>MRTIHANSSAVREDHRALDVATELAKTFRVTVRERERAGGTPKAERDAIRRSGLLTLLISKERGGLGESWPTVYEAIAEIASADASLGHLFGYHFSNFAYVDLFASPEQKARWYPQAVRERWFLGNASSENNAHVLDWRVTATPLPDGSYEINGTKAFCSGSADADRLLVFAVTSRDPNGDGRIVAALIPSDRAGVQVNGDWDSLGMRQTDSGSVTFSGVVVYPDELLGTPGQVTDAFASGSKPSLWTPITQLIFTHLYLGIARGALEEAAHYSRSHSR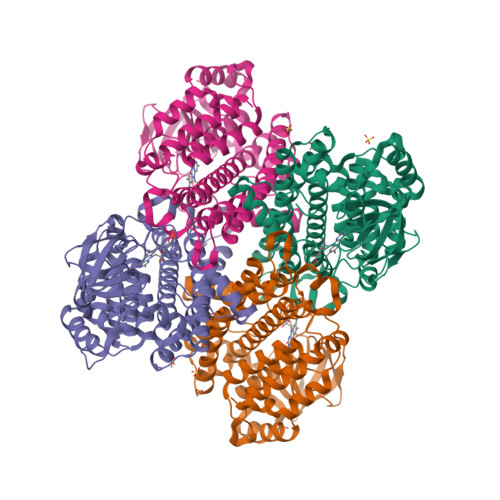PFTLAGVEKATEDPYVLAIYGEFAAQLQVAEAGAREVALRVQELWERNHVTPEQRGQLMVQVASAKIVATRLVIELTSRLYEAMGARAAASRQFGFDRFWRDARTHTLHDPVAYKIREVGNWFLNHRFPTPSFYS[4x]> EFNPYQKGPDPTASALERNGPFAIRSTSVSRTSVSGFGGGRLYYPTASGTYGAIAVSPGFTGTSSTMTFWGERLASHGFVVLVIDTITLYDQPDSRARQLKAALDYLATQNGRSSSPIYRKVDTSRRAVAGHAMGGGGSLLAARDNPSYKAAIPMAPWATSSTAFRTVSVPTMIFGCQDDSIAPVFSSAIPIYNAIPNSTRKNYVEIRNDDHLCVMNGGGHDATLGKLGISWMKRFVDNDTRYSPFVCGAEYNRVVSSYEVSRSYNNCPY

Substituting His/Phe with Ser/Ile should expand the substrate-binding pocket to accommodate the bulkier substrate PET, and the strategy termed “double mutation (DM)” has proven to be useful to enhance PET hydrolytic activity of several IsPETase-like enzymes. Here, we report our experience in establishing the P. pastoris strain that expresses a PET hydrolytic enzyme from Caldimonas taiwanensis termed CtPL-DM that was identified from sequence mining from GenBank and modified by the DM strategy. In contrast to the protein expressed in Escherichia coli, CtPL-DM expressed in P. pastoris is inactive in PET degradation. Structural analysis indicates that a putative N-glycosylation site N181 could restrain the conformational change of a substrate-binding Trp and hamper the enzyme action.

We thus constructed N181A to remove the N-glycosylation and found that the PET hydrolytic activity of this variant was restored. The performance of N181A was further enhanced via molecular engineering. PET hydrolytic activity measurement indicates that F235L and CC are the most promising variants, whose activity was elevated by more than 60% and ~ 20% activity at 60 ºC, respectively. The crystal structure of the inactive variant of F235L, termed F235L-S155A, was successfully solved, which shares a highly identical overall fold to those of CtPL-DM and CtPL-DM-S155A. Since the attempt to obtained substrate/analogue-bound complex failed, the MHET in IsPETase/MHET complex structure was modeled into these apo-form structures to investigate their substrate-binding modes. Compared with two DM structures, the cavity in the rear of the MHET in F235L-S155A is slightly expanded, which might create a broader substrate-binding tunnel to facilitate the binding of PET. This is similar to that was observed in the complex structure of LCC-ICCG and should be considered as a factor to render the higher activity. In addition to the substrate-binding tunnel, the structure of F235L-S155A also provides an opportunity to visualize the N181A-mediated effects. In all three structures, the TPA-binding W180 adopts conformations that should collide with the MHET. Nonetheless, W180 in F235L-S155A, which carries N181A mutation, shall be able to wobble freely.>MAEQKSSNGGGGGGDVVINVPVEEASRRSKEMASPESEKGVPFSKSPSPEISKLVGSPNKPPRAPNQNNVGLTQRKSFARSVYSKPKSRFVDPSCPVDTSILEEEVREQLGAGFSFSRASPNNKSNRSVGSPAPVTPSKVVVEKDEDEEIYKKVKLNREMRSKISTLALIESAFFVVILSALVASLTINVLKHHTFWGLEVWKWCVLVMVIFSGMLVTNWFMRLIVFLIETNFLLRRKVLYFVHGLKKSVQVFIWLCLILVAWILLFNHDVKRSPAATKVLKCITRTLISILTGAFFWLVKTLLLKILAANFNVNNFFDRIQDSVFHQYVLQTLSGLPLMEEAERVGREPSTGHLSFATVVKKGTVKEKKVIDMGKVHKMKREKVSAWTMRVLMEAVRTSGLSTISDTLDETAYGEGKEQADREITSEMEALAAAYHVFRNVAQPFFNYIEEEDLLRFMIKEEVDLVFPLFDGAAETGRITRKAFTEWVVKVYTSRRALAHSLNDTKTAVKQLNKLVTAILMVVTVVIWLLLLEVATTKVLLFFSTQLVALAFIIGSTCKNLFESIVFVFVMHPYDVGDRCVVDGVAMLVEEMNLLTTVFLKLNNEKVYYPNAVLATK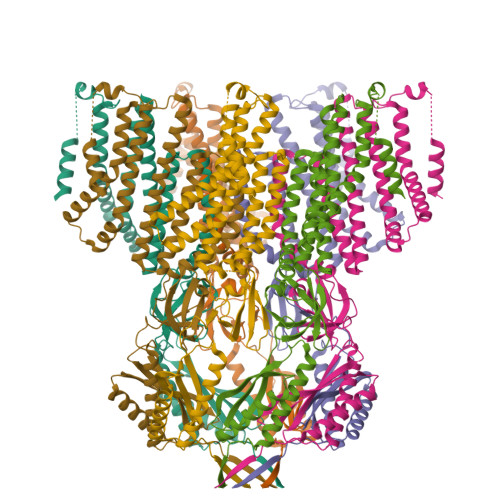PISNYFRSPNMGETVEFSISFSTPVSKIAHLKERIAEYLEQNPQHWAPVHSVVVKEIENMNKLKMALYSDHTITFQENRERNLRRTELSLAIKRMLEDLHIDYTLLPQDINLTKKNSLEVLFQ[7x]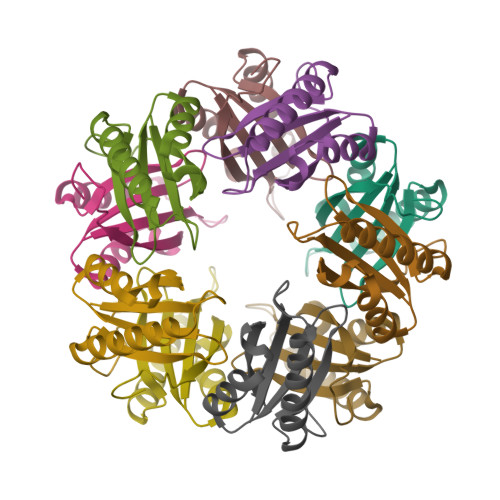>[20x]MLYLVRMTVNLPRNLDSREEERLKASEKARSRTLQEQGQWRYLWRTTGKYGNISVFDVNSHDELHEILWSLPFFPYLTIDVEPLSHHPARVGKD>GMSSSGTSITCEVGLQLIVPDRAPVPLVARLDYSVDDPYAIRAAFHVGDDEPVEWIFARELLTVGIIRETGEGDVRIWPSQDGKERMVN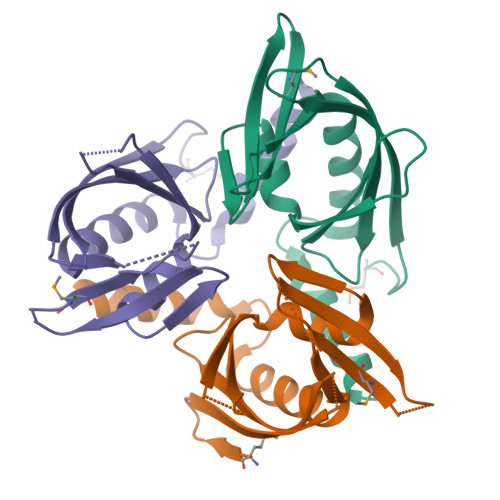IALSSPFGQARFHAQVAPLSEFLHRTYELVPAGQESDYIDIDAEIAEHLS[3x]> PRADEFDTLREKYKAMLNGGTTYNLSDPDIAARVNAITVTAQGYWDSMLKDPNRNRLWNDAPFGSDSTSITTTYRHLYDMALAYTTYGSSLQGNAALKADIISGLDWMNANQFYNGCSQYQNWWHWQIGGPMALNDIVALMYTELTATQISNYMAAIYYTQA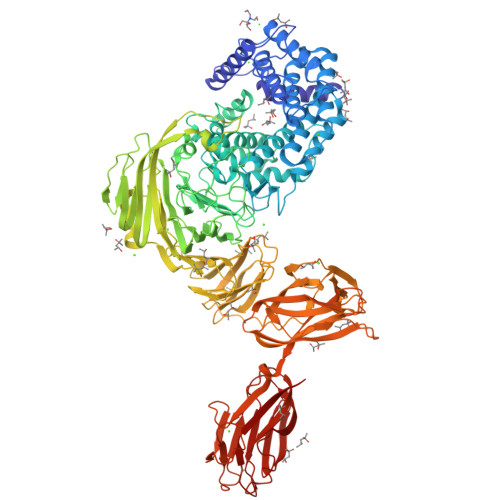SVTMTGANRLWESQVIAISGILNKDSARVAAGRDGISALLPYVAKGDGFYNDGSFVQHTYYAYNGGYGSELLSGIADLIFILNGSSWQVTDPNKNNVYRWIYDSYEPFIYKGNLMDMVRGREISRHGLQDDKAAVTVMASIIRLSQTAASADATAFKRMVKYWLLLDTDKTFLKAVSIDLIIAANQLVNDSTVTSRGELVKYKQFSGMDRAVQLRPGFGFGLSMFSSRIGNYESINAENNKGWHTGDGMTYLYNTDLSQFNDHFWATVDNYRLPGTTVLQNTTQTANSRSDKSWAGGTDILGQYGVSGMELHTVGKSLTAKKSWFMFDDEIVALGSGIASTDGIATETIVENRKLNSSGNNALIVNGTAKPGSLGWSETMTGTNYIHLAGSVPGSDIGYYFPGGAAVKGLREARSGSWSSLNSSASWKDSTLHTRNFMTLWFDHGMNPTNGSYSYVLLPNKTSSAVASYAATPQISILENSSSAQAVKETQLNVTGINFWNDEPTTVGLVTSNRKASVMTKETASDFEISVSDPTQSNVGTIYIDVNKSATGLISKDNEITVIQYYPTMKFKVNVNNSGGKSYKVKFSLTGTPGSNPSPIPIPNPYEAEALPINALTDTPVVYNDANASGGKKLGFNNNAVDDYVEFSLDVTQPGTYDVKSRIMKSTNSGIYQLSINGTNVGSAQDMFWTTSELSKEFTMGSYSFTSPGSYLFRLKTTGKNVSSSGYKLMLDNFSLVSTGIDTTVIVDNADAAGVTKVGTWTGTNTQTDRYGADYIHDGNTGKGTKSVTFTPNVPISGTYQVYMMWAAHTNRATNVPVDVTHSGGTATLNVNQQGNGGVWNLLGTYSFNAGSTGAIKIRTDATNGYVVADAVKLVKVP> AGA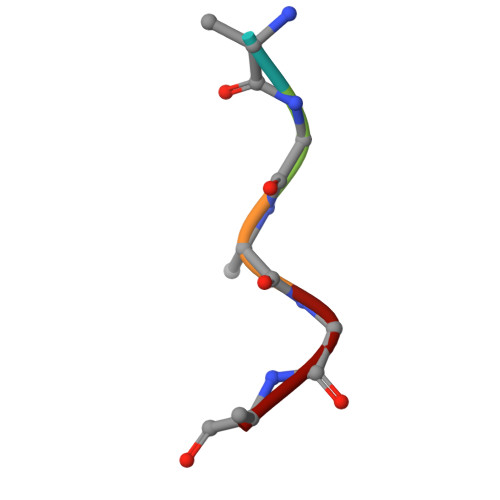GA>[15x]GDNQDRTVANTQPSGPSNSTEIPALTAVETGHTSQVDPSDTIQTRHVVNFHSRSESTIENFMGRAACVFMDQYKINGEETSTDRFAVWTINIREMAQLRRKCEMFTYMRFDIEMTMVITSCQDQGTILDQDMPVLTHQIMYVP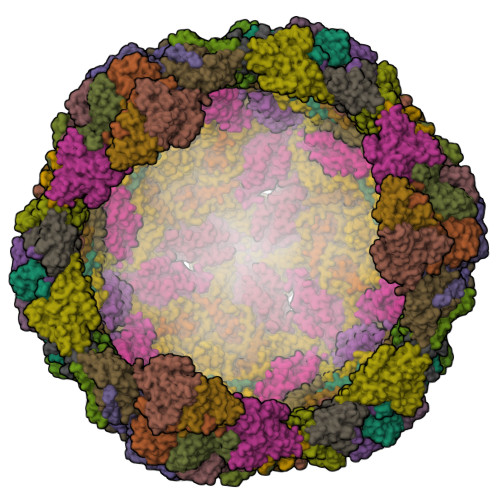PGGPIPAKVDGYEWQTSTNPSVFWTEGNAPPRISIPFISVGNAYSSFYDGWSHFTQDGTYGYTTLNAMGKLYIRHVNRSSPHQITSTIRVYFKPKHIKAWVPRPPRLCPYINKRDVNFVVTEITDSRTSITDTPHPEHSVLATH;>[15x]SPSAEECGYSDRVRSMTLGNSTITTQESANVVVGYGEWPSYLSDREATAEDQPTQPDVATCRFYTLESVQWEKTSPGWWWKFPEALKNMGLFGQNMHYHYLGRAGYTIHVQCNASKFHQGCLLVVCVPEAEMGCADTDTTFPATELTTEDTPHVFTSDSITGKKVQAAVCNAGMGVGVGNLTIFPHQWINLRTNNSATIVIPYINSVPMDNMFRHYNFTLMIIPFAPLNFTDGATAYVPITVTIAPMYAEYNGLRLASTQ;>[15x]GVPVLNTPGSNQFLTSDDYQSPSAMPQFDETPEMHIPGEVRNLMEIAEVDSVVPVNNVTGKTKSMDAYQIPVGTGNTDKTKPIFSFQMDPGYSSVLKRTLLGEMLNYYAHWSGSVKLTFLFCGSAMATGKLLISYSPPGASVPTSRKDAMLGTHIVWDIGLQSSCVLCVPWISQSHYRMVQQDPYTSAGYITCWYQTNIVVPPGAPTSCDVLCFASACNDFSVRLLRDTPFMAQPGKLQ> IVGGQECKDGECPWQALLINEENEGFCGGTILSEFYILTAAHCLYQAKRFKVRVGDRNTEQEEGGEAVHEVEVVIKHNRFTKETYDFDIAVLRLKTPITFRMNVAPACLPERDWAESTLMTQKTGIVSGFGRTHEKGRQSTRLKMLEVPYVDRNSCKLSSSFIITQNMFCAGYDTKQEDACQGDSGGPHVTRFKDTYFVTGIVSWGEG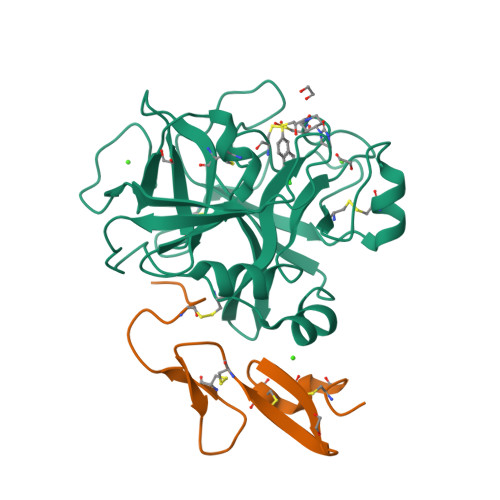CARKGKYGIYTKVTAFLKWIDRSMKTRGLPKAK;> GRARKLCSLDNGDCDQFCHEEQNSVVCSCARGYTLADNGKACIPTGPYPCGKQTLER> MSLKRRQTNIIGVYLADYGGSFYGELLEGIKKGLALFDYEMIVCSGKKSHLFIPEKMVDGAIILDWTFPTKEIEKFAERGHSIVVLDRTTEHRNIRQVLLDNRGGATQAIEQFVNVGSKKVLLLSGPEKGYDSQERLAVSTRELTRFGIPYEIIQG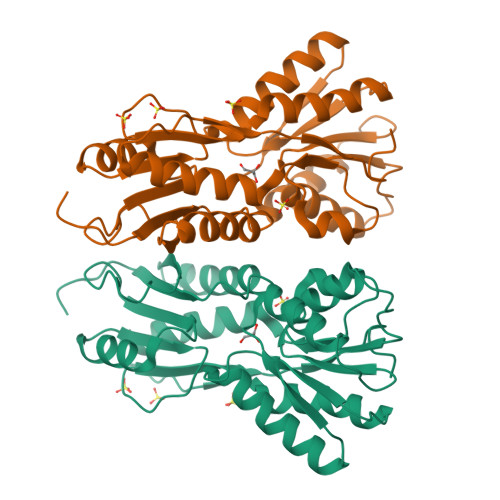DFTEPSGYAAAKKILSQPQTEPVDVFAFNDEMAIGVYKYVAETNYQMGKDIRIIGFDNSELGAFVQPRLATIAYSKHRWGMVAAEKIIHLMRGEAAESEHIYTRFIEGESFPSEGHHHHHH>[2x]SNASNAVKRKGVEVIIALDISNSMLAQDVQPSRLEKAKRLISRLVDELDNDKVGMIVFAGDAFTQLPITSDYISAKMFLESISPSLISKQGTAIGEA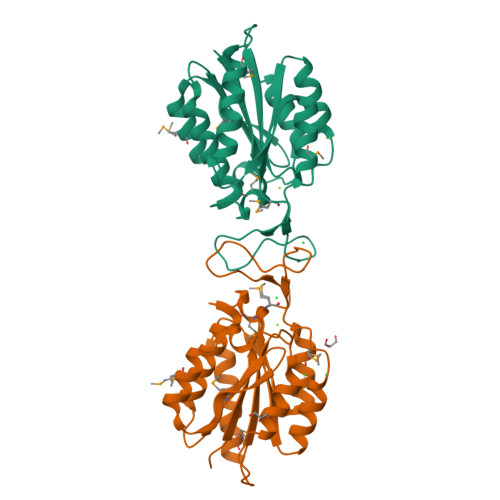INLATRSFTPQEGVGRAIIVITDGENHEGGAVEAAKAAAEKGIQVSVLGVGMPEGAPIPVEGTNDYRRDREGNVIVTRLNEGMCQEIAKDGKGIYVRVDNSNSAQKAISQEISKMAKSDVE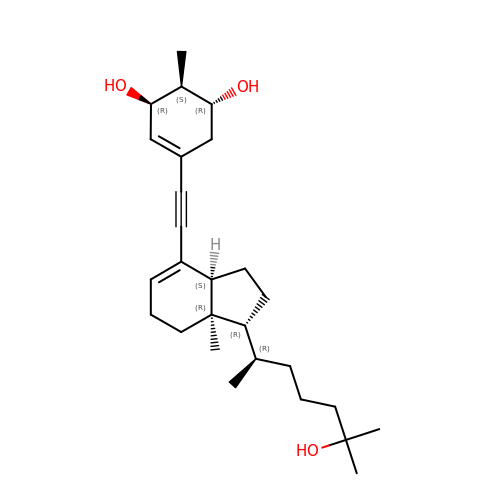(1R,2S,3R)-5-[2-[(1R,3aS,7aR)-1-[(2R)-6-hydroxy-6-methyl-heptan-2-yl]-7a-methyl-1,2,3,3a,6,7-hexahydroinden-4-yl]ethynyl]-2-methyl-cyclohex-4-ene-1,3-diol | C27 H42 O3 | YCBJWNMIMDLOPD-ADFBMCJESA-N>[4x]SNAMKHMEKFANHFGYNRMFAKDQLTLGVHIPIENYQFHAPTMEKQVELVQKAEQYGFTGVWLRDVLLQDPDFGDPATGQIYDMMIYLTYLASK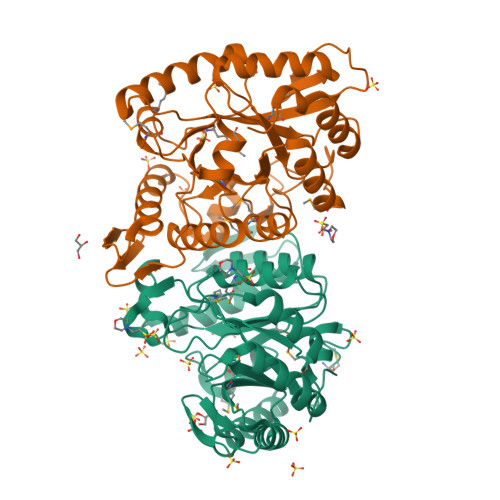TEKIAFGTSATVLSLRHPLRVAKEIATLDQLFPERIMLGVSSGDRRADFKALGVSHETRGEKFREAFAYLEEILYKNFPSIQSTLGEVHGANLVPKPSKRVPTFITGFSQQNMEWFAEHGDGWMYYPRSPVHQAGAIGQWRELVEDYHPDVFKPFIQPMHLDLSEDPNERPTPIRLGYRTGRKALIELLDIYKSIGVNHLFLALFDGQRPADEVLDELGEEVLPHFPAL>[6x]AQQMPSLAPMLEKVMPSVVSINVEGSTTVNTPRMPRNFQQFFGDDSPFCQEGSPFQSSPFCQGGQGGNGGGQQQKFMALGSGVIIDADKGYVVTNNHVVDNATVIKVQLSDGRKFDAKMVGKDPRSDIALIQIQNPKNLTAIKMADSDALRVGDYTVAIGNPFGLGETVTSGIVSALGRSGLNAENYENFIQTDAAI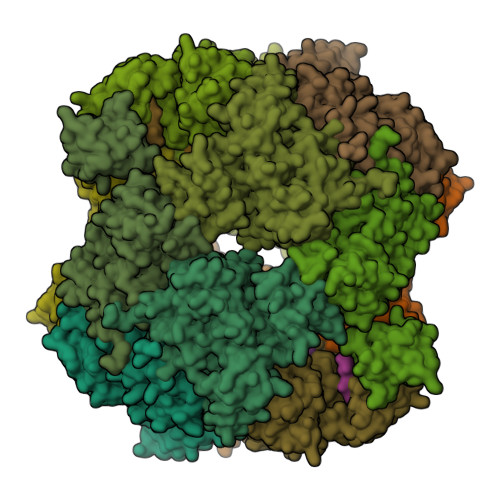NRGNAGGALVNLNGELIGINTAILAPDGGNIGIGFAIPSNMVKNLTSQMVEYGQVKRGELGIMGTELNSELAKAMKVDAQRGAFVSQVLPNSSAAKAGIKAGDVITSLNGKPISSFAALRAQVGTMPVGSKLTLGLLRDGKQVNVNLELQQSSQNQVDSSSIFNGIEGAEMSNKGKDQGVVVNNVKTGTPAAQIGLKKGDVIIGANQQAVKNIAELRKVLDSKPSVLALNIQRGDSTIYLLMQ;>[12x]CYRKL2-ethyl-2-(hydroxymethyl)-N-(6-methylpyridin-3-yl)butanamide | C13 H20 N2 O2 | 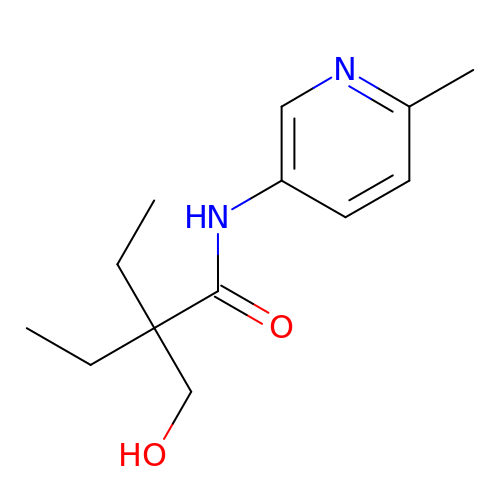FUZYSBUZNYZZBN-UHFFFAOYSA-N> DMPVERILEAELAVEPKTETYVEANMGLNPSSPNDPVTNICQAADKQLFTLVEWAKRIPHFSELPLDDQVILLRAGWNELLIASFSHRSIAVKDGILLATGLHVHRNSAHSAGVGAIFDR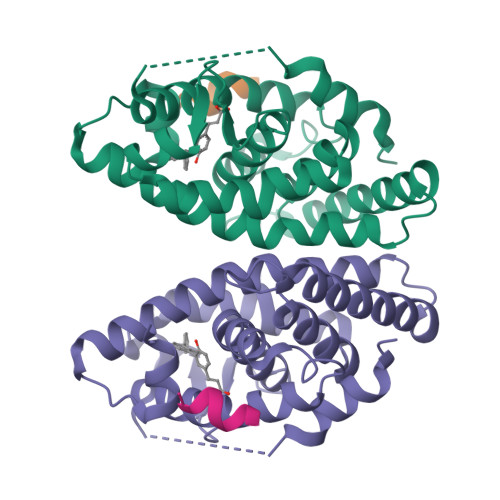VLTELVSKMRDMQMDKTELGCLRAIVLFNPDSKGLSNPAEVEALREKVYASLEAYCKHKYPEQPGRFAKLLLRLPALRSIGLKCLEHLFFFKLIGDTPIDTFLMEMLEA;> KILHRLLQ> LERTIEERVNILFDFVKKKKEEGVIDSSDKEIVAEAERLDVKAMGPLVLTEVLFNEKIREQIKKYRRHFLRFC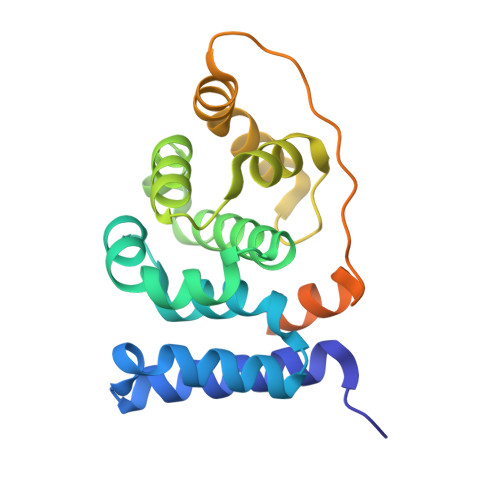HNNKKAQRYLLHGLECVVAMHQAQLISKIPHILKEMYDADLLEEEVIISWSEKASKKYVSKELAKEIRVKAEPFIKWLKEAEEESSGGEEEDEDENIEVVYSKLESVPKVETVKSDNKDDDIDIDAILEHHHHHH> GSMAEGSAVSDPQHAARLLRALSSFREESRFCDAHLVLDGEEIPVQKNILAAASPYIRTKLNYNPPKDDGSTYKIELEGISVMVMREILDYIFSGQIRLNEDTIQDVVQAADLLLLTDL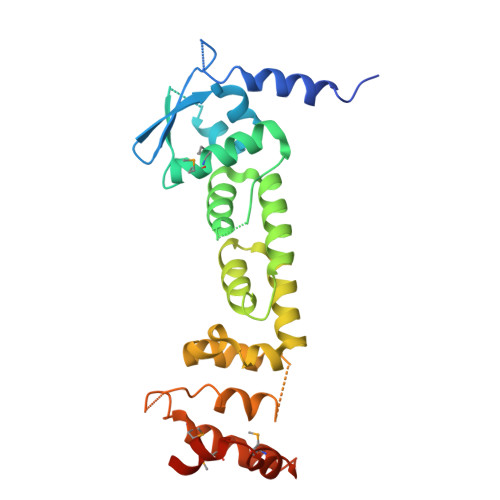KTLCCEFLEGCIAAENCIGIRDFALHYCLHHVHYLATEYLETHFRDVSSTEEFLELSPQKLKEVISLEKLNVGNERYVFEAVIRWIAHDTEIRKVHMKDVMSALWVSGLDSSYLREQMLNEPLVREIVKECSNIPLS> ADTLLILGDSLSAGYRMSASAAWPALLNDKWQSKTSVVNASISGDTSQQGLARLPA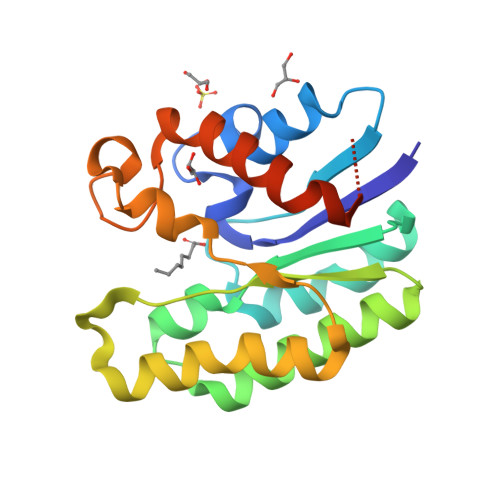LLKQHQPRWVLVELGGNDGLRGFQPQQTEQTLRQILQDVKAANAEPLLMQIRLPANYGRRYNEAFSAIYPKLAKEFDVPLLPFFMEEVYLKPQWMQDDGIHPNRDAQPFIADWMAKQLQPLVNHDSLEHHHHHH>NKTHQVEHESEQSDFQDIRFGLNSVKLPKAQPAAATRITVENGTDKLVNYKSSPQQLFLAKNALKDKLQGEFDKFLSDAKAFPALTADLQEWVDQQLFNPNQSFFDLSAPRSNFTLSSDKKASLDFIFRFTNFTESVQLLKLPEGVSVVVDSKQSFDYYVNASAQKLLVLPLSLPDYTLGLNYMFDHITLNGKVVNKFSFNPFKTNLNLAFSNVYNGVDVFEAQKNLVGKGKYLNTHVKAEDVKKDVNANIKNQFDIAKIIAELMGKALKEFGNQQEGQPLSFLKVMDKVKEDFEKLFNLVRPGLGKFVKDLIQSSSQAENKITVYKLIFDNKKTILNLLKELSIPELNSSLGLVDVLFDGITDSDGLYERLQSFKDLIVPAVKTNEKTAALSPLIEELLTQKDTYVFDLIQKHKGILTNLLKNFLADFQKSTPFMADQVAIFTELFDNEGAFDLFGEADFVDKIAELFLTKRTVKNGEKIETKDSLLVTSLKSLLGEKVAALGDLLDSYIFKNELLNRSVEVAKAEAKDTKGATDYKKEQAKALKKLFKHIGENTLSKTNLDKITLKEVKNTENVELEETETTLKVKKLDVEYKVELGNFEIKNGLIKAMLEFLPDTKDLETTLDKLLFKGESYKAMKDKYIKEGFPGYGWAKGVVPGAFESIENTFKSAIDKTKSIRDLFGDMLFGNDLSSVKETDSFITLGGSFDIKYGGENLNVLPAYYSLINSEIGYQIIGVDTTIDATKVKVELKNKEYKGKSPAINGQVKLSQSFFNVWTNMFDSITKQIFQKKYEFKDNIQVFARNEDNTSRLELDISDPEQRVIPFAFVDGFGIQLKAVDKNITKEAGNTEPKSPVIQLYEALNKEKDQKQQSKQSPKQLDTKTQLGYLLKLGDNWSKDDYKSLIDDTIINNNYLEASFNSKITVDRLGIPIDLWLFKIWPKFNLEIPMQGSLQLYSSSVIFPYGIYDTSVQDAAKIVKRLNFTDMGFKLNDPKPNFWFVGFKHHHHH[2x]

Here, we report a comprehensive structural and functional analysis of the previously uncharacterized protein P116 (MPN_213). Single-particle cryo-electron microscopy of P116 reveals a homodimer presenting a previously unseen fold, forming a huge hydrophobic cavity, which is fully accessible to solvent. Lipidomics analysis shows that P116 specifically extracts lipids such as phosphatidylcholine, sphingomyelin and cholesterol. Each monomer consists of two distinct domains: the core domain (residues 246–867) and the amino-terminal domain (residues 60–245), situated distal to the dimer axis.

The core domain resembles a half-opened left hand, with four contiguous antiparallel pairs of amphipathic α-helices corresponding to the four fingers and the N-terminal domain corresponding to the thumb. The dimer interface, which corresponds to the wrist, is composed of helices with a conserved tryptophan residue (Trp681) that interacts tightly with the neighboring monomer. The palm of the hand includes a long and well-defined central α-helix, namely the bridge helix (residues 268–304), and a rigid β-sheet of five antiparallel strands that extends to the N-terminal domain. The core domain forms a large cavity that measures 62 Å from the proximal to the distal end and 38 Å from the anterior to the posterior side. The cavity has a volume of ~18,000 Å3. The cavity is completely hydrophobic but is fully accessible to the solvent. For the inner part of the P116 core domain, the cryoEM maps show prominent elongated densities (with a length of 10–19 Å and a width of 4 Å) that fill most of the hydrophobic areas. Instead, the mass excess of ~13 kDa, consistently measured by multiple angle light scattering (MALS) and mass spectrometry for P116 in different preparations, could be explained by the presence of ligand molecules bound to P116.As the first reported host of “non-pathogenic-derived” pili, Lactobacillus rhamnosus GG is a gut-adapted commensal lactic acid bacterium (LAB) and one of many clinically investigated probiotic strains for human use in the prevention and treatment of certain gastric ailments. As with other Gram-positive bacteria, sortase-dependent piliation in L. rhamnosus GG (called SpaCBA) is assembled from the ~30 kDa SpaA (backbone), ~20 kDa SpaB (basal), and ~90 kDa SpaC (tip-located) pilins. Two immunoglobulin (Ig)-like subdomains comprise GG-SpaA, each having the conserved residues of a canonical E-box motif and internal isopeptide bonds formed between either lysine and asparagine or lysine and aspartate residues. Our findings show that the GG-SpaA structure has certain features in common with other pathogen-derived pilin-proteins, such as the Ig-like CnaB-type folds and the presence of internal isopeptide bonds6940.

As an alternative, GG-SpaA protein was fragmented by limited proteolysis as had been done previously for other backbone pilins. This produced a 15 kDa-sized fragment that can be crystallized in two different forms. Whereas the tetragonal crystals had diffracted to 2.0 Å and 1.6 Å resolution at home and synchrotron sources, respectively, the orthorhombic crystals showed diffraction to 2.0 Å resolution at both sources. In parallel, we solved the crystal structure of the tetragonal form with an advanced molecular replacement program using search models from distant homologs. As a pruned search template, the C-terminal domain of the S. agalactiae GBS52 pilin4 yielded an interpretable electron-density map for model building, though it offered less than 20% sequence identity. Refined models for the tetragonal and orthorhombic crystals (residues 176–298) gave Rwork/Rfree values of 13.9%/15.8% and 21.6%/24.9%, respectively. The structure of a 15 kDa fragment of GG-SpaA that had been generated by limited proteolysis is identical to that of the C-domain of full-length GG-SpaA (see preceding section for details). However, the electron density for the residues belonging to the extended C-terminal tail was not observed, with proteolytic removal as the likely reason.

> MGRDPNSTNDTTTQNVVLTKYGFDKDVTAIDRATDQIWTGDGAKPLQGVDFTIYNVTANYWASPKDYKGSFDSAPVAATGTTNDKGQLTQALPIQSKDASGKTRAAVYLFHETNPRAGYNTSADFWLTLPAKAAADGNVYVYPKNVQKTTYERTFVKKDAETKEVLEGAGFKISNSDGKFLKLTDKDGQSVSIGEGFIDVLANNYRLTWVAESDATVFTSDKSGKFGLNGFADNTTTYTAVETNVPDGYDAAANTDFKADNSSSDILDAPSGILPLEHHHHHH> MRMLSRNATFNSHGQDSSYFLGWQEYEKNPYHEVHNTNGIIQMGLAENQLCFDLLESWLAKNPEAAAFKKNGESIFAELALFQDYHGLPAFKKAMVDFMAEIRGNKVTFDPNHLVLTAGATSANETFIFCLADPGEAVLIPTPYYPGFDRDLKWRTGVEIVPIHCTSSNGFQITETALEEAYQEAEKRNLRVKGVLVTNPSNPLGTTMTRNELYLLLSFVEDKGIHLISDEIYSGTAFSSPSFISVMEVLKDRNCDENSEVWQRVHVVYSLSKDLGLPGFRVGAIYSNDDMVVAAATKMSSFGLVSSQTQHLLSAMLSDKKLTKNYIAENHKRLKQRQKKLVSGLQKSGISCLNGNAGLFCWVDMRHLLRSN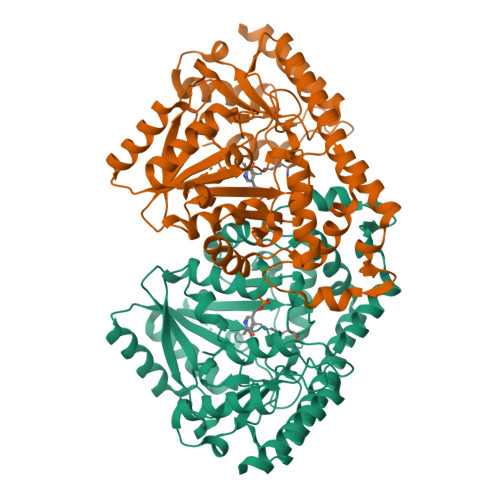TFEAEMELWKKIVYEVHLNISPGSSCHCTEPGWFRVCFANLPERTLDLAMQRLKAFVGEYYNV> MKHHHHHHHHGGLVPRGSHGGSMENNSLAPLRVGILGFGGLGQAAARLLAPKQEMKLVAVADRHGYLYDADGIDVDNAVQAYTQQGSVGKAKKGQMSEQSIEDLIGEGEVDGYFLALPNLPNTFMADVTRQFIASGWQGVLVDALKRTSAVEQLITLREDLAQAGITYMTGCGATPGLLTAAAAIASQSFQEIHQVKITFGVGIANWEAYRATIREDIAHMPGYNVDKAQAMTDAEVAALLDQTNGILALEDMEAADDIMLELAGICHRDQVTVGGVVDTRNPKKPLSTHV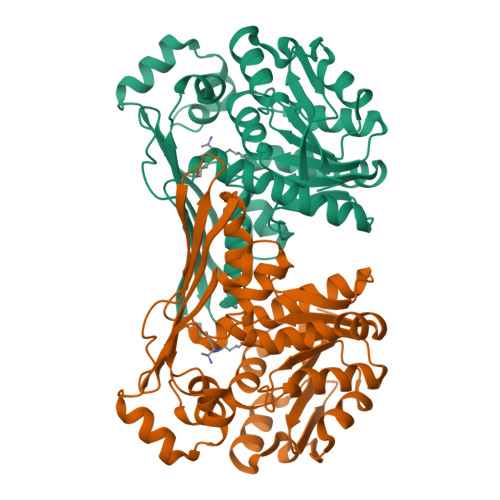KITGRTFEGKISSHTFTLGDETSMAANVCGPAFGYLKAGYGLHRQGLKGLFTAADVMPKFVR>SRAPAPATPHAPDHSPAPNSPTLTRPPEGPKFPRVKNWELGSITYDTLCAQSQQDGPCTPRRCLGSLVLPRKLQTRPSPGPPPAEQLLSQARDFINQYYSSIKRSGSQAHEERLQEVEAEVASTGTYHLRESELVFGAKQAWRNAPRCVGRIQWGKLQVFDARDCSSAQEMFTYICNHIKYATNRGNLRSAITVFPQRAPGRGDFRIWNSQLVRYAGYRQQDGSVRGDPANVEITELCIQHGWTPGNGRFDVLPLLLQAPDEAPELFVLPPELVLEVPLEHPTLEWFAALGLRWYALPAVSNMLLEIGGLEFSAAPFSGWYMSTEIGTRNLCDPSRYNILEDVAVCMDLDTRTTSSLWKDKAA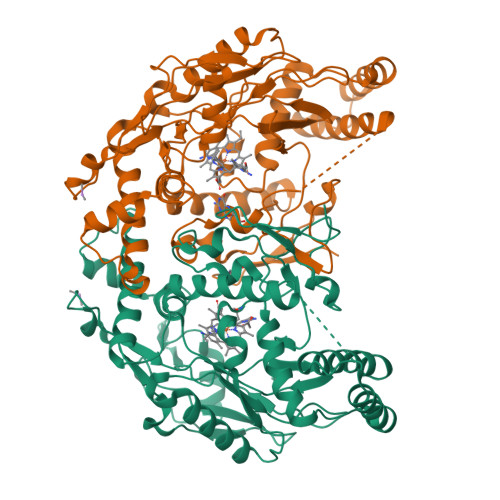VEINLAVLHSFQLAKVTIVDHHAATVSFMKHLDNEQKARGGCPADWAWIVPPISGSLTPVFHQEMVNYILSPAFRYQPDPW[2x]N,N'-(butane-1,4-diyl)bis(N-{3-[(2,3-dihydroxybenzene-1-carbonyl)amino]propyl}-2,3-dihydroxybenzamide) 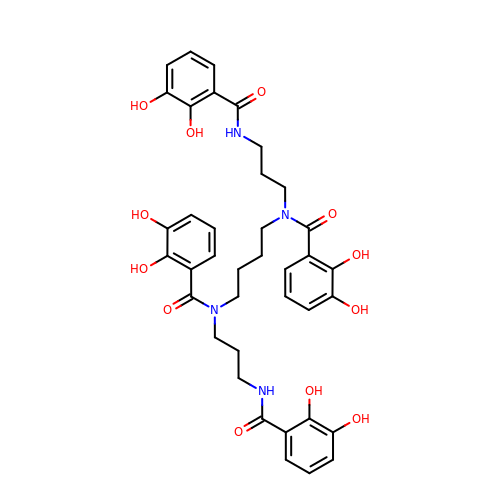| C38 H42 N4 O12 | WNIXXCINEMCWIS-UHFFFAOYSA-N> MQPINTSNPDNTASYVKDEVEITSSTIALSEIVSVVNTSDGRLEVFGVGTDKAVWHNRQMAPHTGSPWSGWSSLKGQVTSKPVVYINTDGRLEVFARGTDNALWHIWQTATNAGWSNWQSLGGVITSNPAIYANTDGRLEVFARGADNALWHISQTTAHSGPWSSWASLNGVITSNPTVHINSDGRLEVFARGTDNALWHIWQTAPDSNLWSSWESLNGIITSDPVVIDTADGRLEVFARGADNALWHIWQTISHSGPWSGWQSLNGVITSAPAVAKNCDNRLEAFARGTDNALWHTWQTVSHSGPWSSWQSLNGVITSAPTAVRDADGRLEVFARGTDNALWLTWQTASSWSPWISLGGVLIDASAIK

PHL, a homo-dimer lectin (~ 80.4 kDa) with subunits linked by a disulfide bridge, was characterized as a dual-specific l-fucose/d-galactose binding protein with an unusually high number of potential binding sites. PHL forms a single domain structure, which exhibits a seven-bladed β-propeller fold organized around a seven-fold pseudoaxis of symmetry. The results of biological activity assays suggest that PHL significantly affects host defense mechanisms, specifically antimicrobial effectors such as reactive oxygen species and their production.

The structure of PHL was solved using the structure of the lectin PLL from Photorhabdus luminescens. Each repeat of the PHL lectin (W-motif) consists of a four-stranded antiparallel β-sheet connected by relatively long loops. The shape of the PHL lectin monomer is a short torus, with a diameter of 45 Å and a height of 30 Å. The tunnel in the center broadens from 13 Å at the C- and N- termini side to a diameter of 18 Å on the opposite side. The overall structure of the PHL monomer is very similar to the recently determined structure of a homologous PLL lectin, with a backbone RMSD of 0.65 Å. The dimeric state of PHL shown by AUC was also seen in the crystal. A pseudo-2-fold axis of symmetry generates the dimer associated in a “tunnel to tunnel” manner, so that the C- and N-termini are exposed to the solvent. The main dimer-stabilizing element is a disulfide bridge formed between the Cys279 residues of both monomers in the loop interconnecting β-strands in repeat W6. Additional hydrogen bonds are formed by residues in the loops of all repeats except W5. Interestingly, site 2F is occupied by the Met60 side chain of the symmetry-related molecule in all structures.>[2x]SGPSGTAAASSSLVSESVVSLAAGTQAVLRCQSPRMVWTQDRLHDRQRVVHWDLSGGPGSQRRRLVDMYSAGEQRVYEPRDRDRLLLSPSAFHDGNFSLLIRA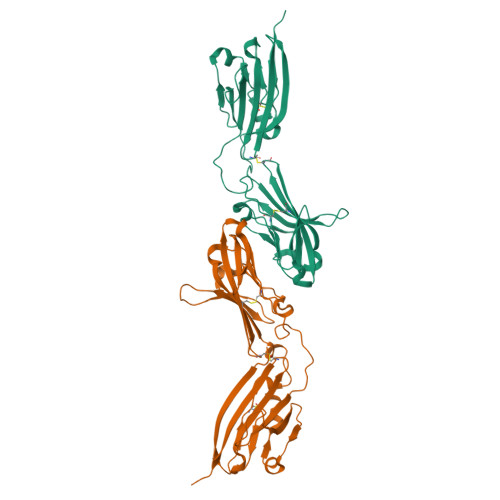VDRGDEGVYTCNLHHHYCHLDESLAVRLEVTEDPLLSRAYWDGEKEVLVVAHGAPALMTCINRAHVWTDRHLEEAQQVVHWDRQLPGVSHDRADRLLDLYASGERRAYGPPFLRDRVSVNTNAFARGDFSLRIDELERADEGIYSCHLHHHYCGLHERRVFHLQVTEPAFE>[2x]GAMEGFKANLSLLRRPGEKTYTQRCRLFVGNLPADITEDEFKRLFAKYGEPGEVFINKGKGFGFIKLESRALAEIAKAELDDTPMRGRQLRVRFATHAAALSVRNLSPYVSNELLEEAFSQFGPIERAVVIVDDRGRSTGKGIVEFASKPAARKAFERCSEGVFLLTTTPRPVIVEPLEQLDDEDGLPEKLAQKNPMYQKERETPPRFAQHGTFEYEYSQRWKSLDEMEKQQREQVEKNMKDAKDKLESEMEDAYHEHQANIL

SFPQ is an RNA- and DNA-binding protein that is involved in many aspects of RNA biogenesis as well as DNA damage repair. The DBHS family proteins share a high sequence similarity within the central DBHS domain which comprises two RNA-recognition motifs (RRMs), a NonA/paraspeckle (NOPS) domain and a long coiled-coil domain. It has previously been shown that SFPQ homo- and hetero-dimerizes via the central DBHS domain and polymerizes via the extended coiled-coil domain, which is critical for its nuclear functions, such as transcriptional regulation and paraspeckle formation. We have previously discovered that SFPQ directly binds to zinc, which promotes the formation of infinite polymers of both the SFPQ homodimers and SFPQ/NONO heterodimers.

Here we characterize two familial ALS (fALS)-associated SFPQ variants, which cause amino acid substitutions in the proximity of the SFPQ zinc-coordinating centre (N533H and L534I). Both mutants display increased zinc-binding affinities, which can be explained by the presence of a second zinc-binding site revealed by the 1.83 Å crystal structure of the human SFPQ L534I mutant. The calculated affinity (IC50) of SFPQ N533H (0.25 µM) and L534I (0.54 µM) binding to zinc was approximately 5.8- and 2.7-fold higher than that of the WT protein (1.45 µM), respectively, confirming that these fALS-associated mutations cause significant increases in SFPQ zinc-binding affinity. The final model consisted of two chains of SFPQ (residues 283–535 in Chain A and residues 290–368, 371–535 in Chain B), two Zn atoms (one of the two with half occupancy), and 277 water molecules. A closer inspection of the two zinc centres showed that the first zinc coordinating centre (Zn centre 1) is almost indistinguishable from that of SFPQ WT, coordinated by His A483, His B530, His A*528 and a carbonyl oxygen of Leu A*535, where the asterisk (*) denotes a symmetry-related dimer (x, y, z – 1). However, the anomalous signal from the second centre (Zn centre 2) is significantly lower than that of Zn centre 1, indicating that this site is not fully occupied. The second zinc coordination centre is composed of three amino acid residues: Glu B*489, Glu B529 and His B*483 (symmetry operator: x, y, z – 1). The side chains of Glu B529 and His B*483 are in the ‘in’ position coordinating zinc, whereas in the absence of zinc, they take on the ‘out’ conformation. Zinc in the second centre is modelled with the occupancy of 0.5 in the final structure with a comparable B-factor value (28.1 Å2) to those ligating atoms (average B-factor of 26.8 Å2). Taken together, the crystal structure of SFPQ L534I in complex with zinc reveals an additional zinc-binding site, providing the structural basis for the apparent increase in zinc-binding affinity in this mutant.> PQQE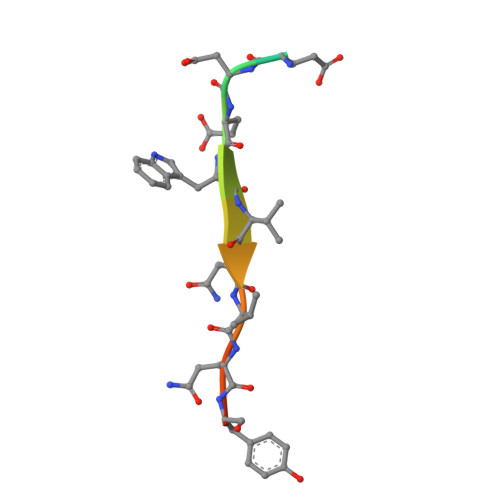DEWVNVQYPD>SKPFTVPILTVEEMTNSRFPIPLEKLFTGPSGAFVVQPQNGRCTTDGVLLGTTQLSPVNICTFRGDVTHIAGTHNYTMNLASQNWNNYDPTEEIPAP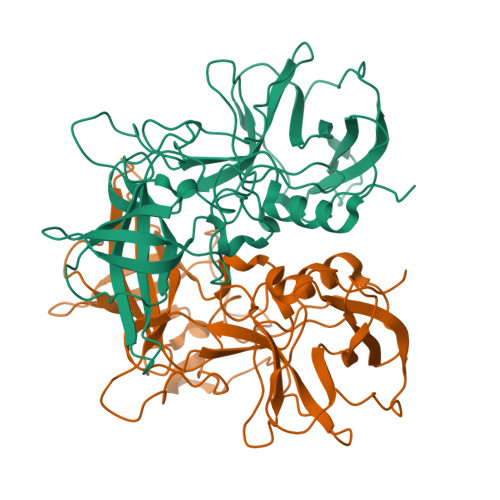LGTPDFVGRIQGMLTQTTRGDGSTRGHKATVSTGDVHFTPKLGSIQFNTDTNNDFETGQNTKFTPVGVVQDGNGAHQNEPQQWVLPSYSGRTGHNVHLAPAVAPTFPGEQLLFFRSTMPGCSGYPNMNLDCLLPQEWVQHFYQEAAPAQSDVALLRFVNPDTGRVLFECKLHKSGYVTVAHTGQHDLVIPPNGYFRFDSWVNQFYTLAPM[2x]We report the functional characterisation of a modified sugar-binding protein, MsBP, from a marine Synechococcus strain, MITS9220. Ligand screening of MsBP shows a specific affinity for zinc (KD ~ 1.3 μM) and a preference for phosphate-modified sugars, such as fructose-1,6-biphosphate, in the presence of zinc (KD ~ 5.8 μM). The presence of the additional C-terminal subdomain places it unambiguously within sub-cluster D-I, associated with a narrow substrate preference for carbohydrates.

The structure of Zn-MsBP showed a single chain containing two Zn2+ atoms in the asymmetric unit (a.s.u). Notably, the structure of Zn-MsBP shows ten molecules of SO42−, possibly sequestered from the sulphate rich crystallisation condition (2 M (NH4)2SO4, 20% w/v PEG3350). One Zn2+ atom (Zn #1) appears at the periphery, weakly held within a negatively-charged cavity of the crystal lattice, created by the side chains of amino acids, such as D87 and T89, from two neighbouring monomers. The second Zn2+ atom (Zn #2) is located within the binding pocket of the protein. However, candidate sidechains in the vicinity include S174, Q227 and R228. The fourth coordination for this zinc may be satisfied with the carboxylate group of D173. This zinc is held peripheral to the binding cleft of the protein and is within 4 Å of the aromatic sidechain of W49, positioned over the binding cleft. Two sulphate ions are positioned in the positively-charged binding cleft: one adjacent to the bound Zn2+ (SO42− #9), and the second buried deeper within the cleft (SO42− #8). In Zn-MsBP, helix 2 is pushed ~ 10 Å over the binding cleft, attenuating access to the substrate-binding channel. The observed partial closure of the binding pocket for Zn-MsBP, caused by the movement of helix 2 exposes a hydrophobic patch to solvent, and positions W49 to occlude the entrance to the cleft, closely positioned to the bound Zn2+. Thus, from the ‘partially-closed’ conformation of the Zn-MsBP structure, it is inferred Zn2+ may modulate ligand binding, consistent with an induced-fit mechanism.

> MGSSHHHHHHSSGLVPRGSMRGSHMPEGTLQLWTLQLAPKFNPYMDDVLGSWDKLHPEALVRWTDLPWGSVERKLLAAVFARTAPDVVNLNPPFAANLASKGGLTDLTALLPPGAEQNYLPSVWEAARDPEAGQIAIPWYLTVRLSLVNGDLLRQAGLSRAPRRWDEVPAYARSIRERTGRYGLFVTVVPDDSAELLESFVQMGVSLLDARQRAAFNTPAGRKAFAFWTDLYREGLLPREVVSQGQRRAIELYQSGELALLASGAEFLRSIQTNAPGVAAVTTPQPPLTGSDGTANVALMTLAVPRQSQQAGEAVELALFLTNGTNQARFAREARVLPSSLEALSAIRAELEVEQPSNPAEAQIRDARLLSAETLNTARVLVPATPGVKRLQSIIYTQLQRAMLGQISSDQAVLEAEQQWNRYASARWP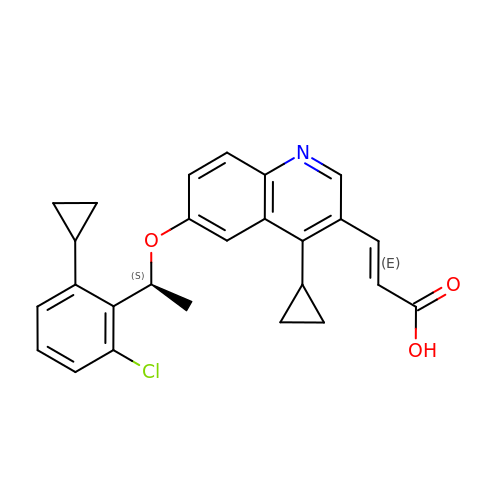(2E)-3-{6-[(1S)-1-(2-chloro-6-cyclopropylphenyl)ethoxy]-4-cyclopropylquinolin-3-yl}prop-2-enoic acid | C26 H24 Cl N O3 | HOMQCLNBKVHZGD-RZXPCSSPSA-N> MRRYNTGLFLLSMVMLAGCGKPEVNVVMTGDMTTRLAFAGEQLKQALVEKGYEVNQTTDEKEIGGGKRSIYLNLLNDTTKKNKERFDISTKGKNTYVTGYDGNGIIYGCRELIDQLDQSGTMDFKPVSDAPEMVLRGACIGLQKTTYLPGHAVYEYPYTPESFPWFYDKERWIKYLDMMVENRMNSLYLWNGHPFASLVKLKDYPFALEVDEETFKKNEEMFSFLTTEAEKRGIFVIQMFYNIIVSKPFADHYGIKTQDRNRPITPLISDYTRKSVAAFIEKYPNVGLLVCLGEAIGTYEEDVEWFTKTIIPGIKDGLKVLGRTDEPPVLVRAHDTDCKMVIDAALPLYKNLYTMHKYNGESLTTYEPRGPWAKIHKDLSSLGSVHISNVHILANLEPWRWSSPDFIQKSVKAMHSVHGANALHIYPQANYWDWPYTADKLANGEREEQVYRDWAWYKAWGRYAWKADRNRLEEIKYWDKQFGDFYGIPAEMADNIRIAYEESGEIAPKLLRRFGITEGNRQTLLLGMFMSQFVNPYKYTIHYGFYESCGPGGEKLIEYVEKEWKKQPHVGELPLDIINQVIEHGDKAVAAIDKVVSSAKKN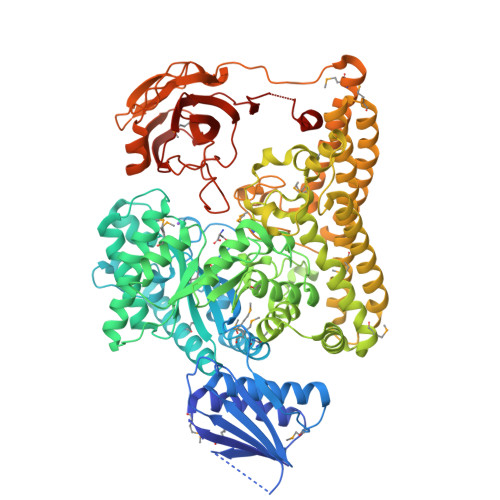SDELRRLQNDMHCYREYAYAFYYKVKAAQHVLNYHWGKNMDELDKAVPLMEESLKHYTKLVDLTKDTYLFANSMQTAQRRIPIGGDDGNNKTWSEMLVHYKAELYNFKENIEMLKDKKVRKCVEVTPLKEADVKILNNLTKVKIEKGAKIFSNIDGGIDAIAKEITGLTGFVFNGEKQRDDATTIEFECSSPVTMLVAYFKDDHRKFAKAPRLESDASANDYGQAEPVLTNALHVKGVALADIYPYKFKAGRHTLILPKGYCGVLGFTEDKIKERDVALEGGADAPDWLFY;> EVNVVMTGDMTTRLAFAGEQLKQALVEKGYEVNQTTDEKEIGGGKRSIYLNLLNDTTKKNKERFDISTKGKNTYVTGYDGNGIIYGCRELIDQLDQSGTMDFKPVSDAPEMVLRGACIGLQKTTYLPGHAVYEYPYTPESFPWFYDKERWIKYLDMMVENRMNSLYLWNGHPFASLVKLKDYPFALEVDEETFKKNEEMFSFLTTEAEKRGIFVIQMFYNIIVSKPFADHYGIKTQDRNRPITPLISDYTRKSVAAFIEKYPNVGLLVCLGEAIGTYEEDVEWFTKTIIPGIKDGLKVLGRTDEPPVLVRAHDTDCKMVIDAALPLYKNLYTMHKYNGESLTTYEPRGPWAKIHKDLSSLGSVHISNVHILANLEPWRWSSPDFIQKSVKAMHSVHGANALHIYPQANYWDWPYTADKLANGEREEQVYRDWAWYKAWGRYAWKADRNRLEEIKYWDKQFGDFYGIPAEMADNIRIAYEESGEIAPKLLRRFGITEGNRQTLLLGMFMSQFVNPYKYTIHYGFYESCGPGGEKLIEYVEKEWKKQPHVGELPLDIINQVIEHGDKAVAAIDKVVSSAKKNSDELRRLQNDMHCYREYAYAFYYKVKAAQHVLNYHWGKNMDELDKAVPLMEESLKHYTKLVDLTKDTYLFANSMQTAQRRIPIGGDDGNNKTWSEMLVHYKAELYNFKENIEMLKDKKVRKCVEVTPLKEADVKILNNLTKVKIEKGAKIFSNIDGGIDAIAKEITGLTGFVFNGEKQRDDATTIEFECSSPVTMLVAYFKDDHRKFAKAPRLESDASANDYGQAEPVLTNALHVKGVALADIYPYKFKAGRHTLILPKGYCGVLGFTEDKIKERDVALEGGADAPDWLFY9-[2-(3,4-dichlorophenyl)ethyl]-2-(3-hydroxyphenyl)-8-oxidanylidene-7~{H}-purine-6-carboxamide 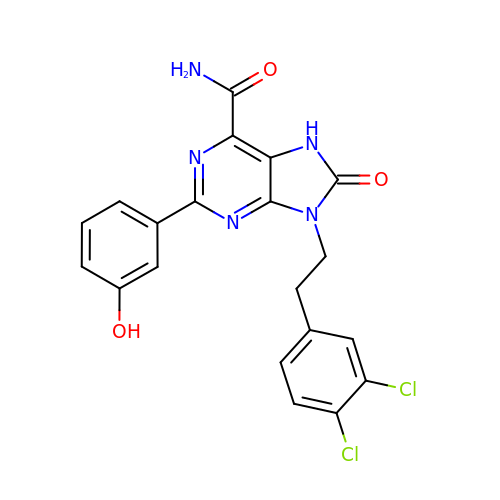| C20 H15 Cl2 N5 O3 | ZOEBAQBSIASRNL-UHFFFAOYSA-N>MSDIFNSPQNKASILTALMKSTTGDVEDVLIPKRFRPAKDPLDSPQAAAQFLKDNKYRILRPRAIPTMVELETDAALPRLRQMVEDGKLKDTVSVPEGTTAFYPKYYPFHKPDHDEVGTFGAPDITLLKQLTFFLLENDFPTGPETLRQVREAIATLQYGSGSYSGQLNRLLAMKGVATGRNPNKTPKTVGYTNEQLAKLLEQTLPINTPKHEDPDLRWAPSWLINYTGDLSTDKSYLPHVTIKSSAGLPYIGKTKGDTTAEALVLADSFIRDLGRAATSADPEAGVKKTITDFWYLSCGLLFPKGERYTQVDWDKKTRNIWSAPYPTHLLLSMVSTPVMNESKLNITNTQTPSLYGFSPFHGGMDRIMTIIRDSLDNDE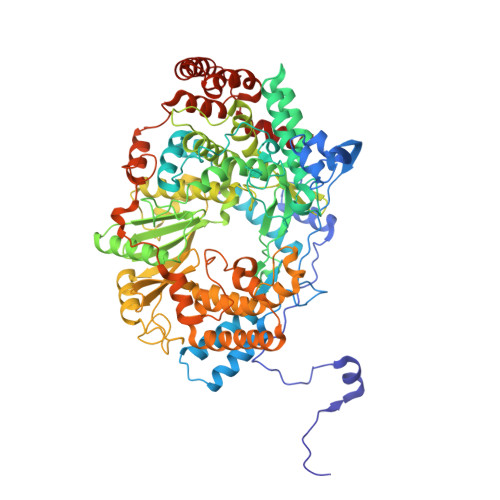DLVMIYADNIYILQDNTWYSIDLEKGEANCTPQHMQAMMYYLLTRGWTNEDGSPRYNPTWATFAMNVAPSMVVDSSCLLMNLQLKTYGQGSGNAFTFLNNHLMSTIVVAEWVKAGKPNPMTKEFMDLEEKTGINFKIERELKNLRETIVEAVETAPQDGYLADGSDLPPIRPGKAVELDLLGWSAIYSRQMEMFVPVLENERLIASAAYPKGLENKALARKPGAEIAYQIVRYEAIRLVGGWNNPLLETAAKHMSLDKRKRLEVKGIDVTGFLDDWNNMSEFGGDLEGITLSEPLTNQTLVDINTPLDSFDPKARPQTPRSPKKTLDEVTTAITSGTYKDPKSAVWRLLDQRTKLRVSTLRDQALALKPASSSVDNWAEATEELAQQQQLLMKANNLLKSSLTETREALEKTGHHHHHH[8x]>ADPKCTVSHEVADCSHLKLTQVPDDLPTNITVLNLTHNQLRRLPAANFTRYSQLTSLDVGFNTISKLEPELCQKLPMLKVLNLQ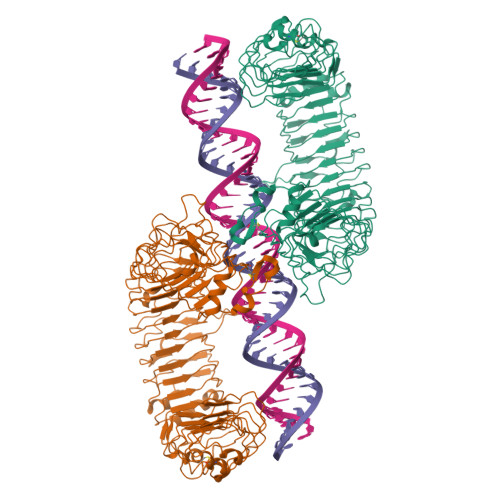HNELSQLSDDTFAFCTNLTELHLMSNSIQKIDNNPFVDQKNLITLDLSHNGLSSTKLGTQVQLENLQELLLSNNKIQALKSEELDIFANSSLKKLELSSNQIKEFSPGCFHAIGRLFGLFLNNVQLGPSLTEKLCLELANTSIRNLSLSNSQLSTTSNTTFLGLKWTNLTMLDLSYNNLNVVGNDSFAWLPQLEYFFLEYNNIQHLFSHSLHGLFNVRYLNLKRSFTKQSISLASLPKIDDFSFQWLKCLEHLNMEDNDIPGIKSNMFTGLINLKYLSLSNSFTSLRTLTNETFVSLAHSPLHILNLTKNKISKIESDAFSWLGHLEVLDLGLNEIGQELTGQEWRGLENIFEIYLSYNKYLQLTRNSFALVPSLQRLMLRRVALKNVDSSPSPFQPLRNLTILDLSNNNIANINDDMLEGLEKLEILDLQHNNLARLWKHANPGGPIYFLKGLSHLHILNLESNGFDEIPVEVFKDLFELKIIDLGLNNLNTLPASVFNNQVSLKSLNLQKNLITSVEKKVFGPAFRNLTELDMRFNPFDCTCESIAWFVNWINETHTNIPELSSHYLCNTPPHYHGFPVRLFDTSSCKSGRLVPRGSHHHHHH[2x]> PISPIETVPVKLKPGMDGPKVKQWPLTEEKIKALVEICTEMEKEGKISKIGPENPYNTPVFAIKKKDSTKWRKLVDFRELNKRTQDFWEVQLGIPHPAGLKKNKSVTVLDVGDAYFSVPLDEDFRKYTAFTIPSINNETPGIRYQYNVLPQGWKGSPAIFQSSMTKILEPFRKQNPDIVIYQYMDDLYVGSDLEIGQHRTKIEELRQHLLRWGLTTPDKKHQKEPPFLWMGYELHPDKWTVQPIVLPEKDSWTVNDIQKLVGKLNWASQIYPGIKVRQLCKLLRGTKALTEVIPLTEEAELELAENREILKEPVHGVYYDPSKDLIAEIQKQGQGQWTYQIYQEPFKNLKTGKYARMRGAHTNDVKQLTEAVQKITTESIVIWGKTPKFKLPIQKETWETWWTEYWQATWIPEWEFVNTPPLVKLWYQLEKEPIVGAETFYVDGAANRETKLGKAGYVTNRGRQKVVTLTDTTNQKTELQAIYLALQDSGLEVNIVTDSQYALGIIQAQPDQSESELVNQIIEQLIKKEKVYLAWVPAHKGIG;> PISPIETVPVKLKPGMDGPKVKQWPLTEEKIKALVEICTEMEKEGKISKIGPENPYNTPVFAIKKKDSTKWRKLVDFRELNKRTQDFWEVQLGIPHPAGLKKNKSVTVLDVGDAYFSVPLDEDFRKYTAFTIPSINNETPGIRYQYNVLPQGWKGSPAIFQSSMTKILEPFRKQNPDIVIYQYMDDLYVGSDLEIGQHRTKIEELRQHLLRWGLTTPDKKHQKEPPFLWMGYELHPDKWTVQPIVLPEKDSWTVNDIQKLVGKLNWASQIYPGIKVRQLCKLLRGTKALTEVIPLTEEAELELAENREILKEPVHGVYYDPSKDLIAEIQKQGQGQWTYQIYQEPFKNLKTGKYARMRGAHTNDVKQLTEAVQKITTESIVIWGKTPKFKLPIQKETWETWWTEYWQATWIPEWEFVNTP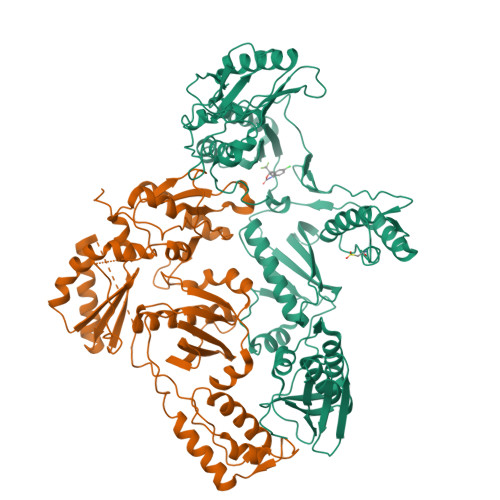PLVKLWYQLEKEPIVGAETF> MAKWVYKFEEGNASMRNLLGGKGCNLAEMTILGMPIPQGFTVTTEACTEYYNSGKQITQEIQDQIFEAITWLEELNGKKFGDTEDPLLVSVRSGARASMPGMMDTILNLGLNDVAVEGFAKKTGNPRFAYDSYRRFIQMYSDVVMEVPKSHFEKIIDAMKEEKGVHFDTDLTADDLKELAEKFKAVYKEAMNGEEFPQEPKDQLMGAVKAVFRSWDNPEAIVYRRMNDIPGDWGTAVNVQTMVFGNKGETSGTGVAFTRNPDTGEKGIYGRYLINAQGEDVVAGVRTPQPITQLENDMPDCYKQFMDLAMKLEKHFRDMQDMEFTIEEGKLYFLQTRNGKRTAPAALQIACDLVDEGMITEEEAVVRIEAKSLDQLLHPTFNPAALKAGEVIGSALPASPGAAAGKVYFTADEAKAAHEKGERVILVRLETSPEDIEGMHAAEGILTVRGGMTSHAAVVARGMGTCCVSGCGEIKINEEAKTFELGGHTFAEGDYISLDGSTG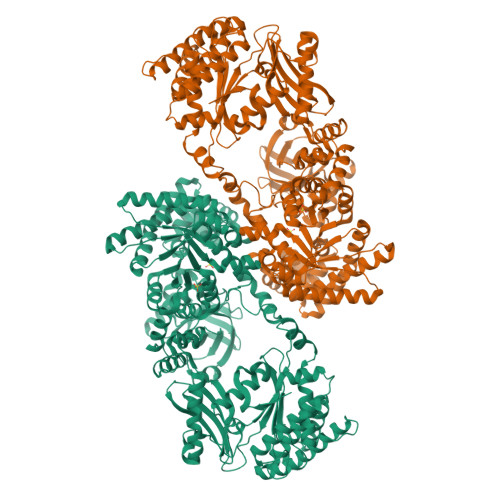KIYKGDIETQEASVSGSFERIMVWADKFRTLKVRTNADTPEDTLNAVKLGAEGIGLCRTEHMFFEADRIMKIRKMILSDSVEAREEALNELIPFQKGDFKAMYKALEGRPMTVRYLDPPLHEFVPHTEEEQAELAKNMGLTLAEVKAKVDELHEFNPMMGHRGCRLAVTYPEIAKMQTRAVMEAAIEVKEETGIDIVPEIMIPLVGEKKELKFVKDVVVEVAEQVKKEKGSDMQYHIGTMIEIPRAALTADAIAEEAEFFSFGTNDLTQMTFGFSRDDAGKFLDSYYKAKIYESDPFARLDQTGVGQLVEMAVKKGRQTRPGLKCGICGEHGGDPSSVEFCHKVGLNYVSCSPFRVPIARLAAAQAALNNK>[2x]MHSTNNNSNKRNNEEKHKQPEIDSSANNGEGTSGTRAQTVGDTATEAGVRNETKAGASTRRQTDGTGLSGTNAKIATASSARQTDVEKPADVTFTIENVDDVGIMQQKKPPTVVQSRTDVFNEQFANEALHPMTKVIFNGLDVNTEVQPLSDDFKQISDPKGYLTYSVKYEDQFTKKDKLRASEADDRIVGPTVNLFKYGAAVVNIDLNRDFFDTATGIDLTKGIPLVQDLLVPIGVTAGAEQSAEYVSGLLMVLFKVMTDNRLVIVGETTTPMSNTLSTVVNNVLRTTYHNNVGVNPALLRDFTQVNWLNRDITNMLQQAGTKYGLGLTETRLDYVRLVKTIVGHALNIDHFAASVLNINLRALMEANVTADDRIKALQAHSMISTQFHGPNQGALRPELAFDHDHIIRCLMLAAANYPRLEGIIVQINTGYVASANVIRPVSEKRYFPENLEQNQSAARLVSAVKARASEADISSIHLAIAREVSPMFNVHELKKIAESFEDPSSIVVVLEFILFALFFPTEFNRIKGDIQNVLLLFFSRWYPVEYGIFIQRGATYTINAAGEFEFSGRNEKWDQSLYLSEHFPALFSDVPLAG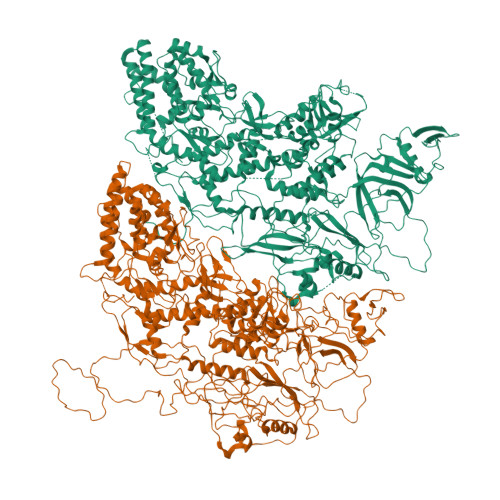ANTIIAIMRLFTPQGFLRTDDLAIAANFPRASRNPQTYIPYTNQRGTVTNEFASRFRTIVATLANVVNERAVQDDMQKATRSCTKQWLRHLETQFDNIAVAHTDHLSVVYATMSNFMLNFTNNFSGNHATFKPDQYVITSPEGSYKPIIERQGETVDGLTIIDTSIVWPILCQCTYPLVRQSGKGVDAVSIMEEIVYPDPSTTLSQSLSVAQVLSKLTLPDAFINMILSGGDSVVMRTYQTEADDDLDEGIRMTTYDQYLSHIRERLHITNVPDPIYITGASTPDQIAASVQATHVAVVLYQSGVINGSASTYLRENEVLVVMPDYYDVVSRFANANLQMNNNRYHESVLEIADIFDQADFIQTSDAVRQLRALMPTLSTSQIRHAIERIAQITDVDSTDYGKLTLRFLGTLTRSLKMQNAQIRRIRPDGTVLRYDDQIDIEAFRWSRYFLDELRLRRLSVGLRLITNPRIARRFDGVRIMYLTDDDPDPDFVPDVPEGYVAVQYAHRLFSSSLANKRNRVTYTHPPTGMAYPSPTGRPHVHMTINERAGMSKLVADNIIASVIKSNWVVDIHDIEYTAEVMTPSEGYTQHVDAESIMTAPKGKLFHLQFMDGLLRPEPSAFDPPASGEDMRLIYPLQPISVARSMRAIVNHNEVDRPRGAVAPSSYEMDTGTLSRNGDLLYSPVANGQVGIPKLEVDHISFSNVVSMMTANIRTGDDMAVERVNPDDVRAINIRNA> GQDEERDVGDDPFVRRAGAFLGIEAGTITIELSNLIDFYIRNGILEMENEQAVYPVNLRGVFDLNILQEMYRQYLIQSFAAKSRTEKERLFNNLAHLGNILGLTSAEVNAIHSNIGSVIYKTYASQALTNNRLEEKDIEFLRNIQNMLSMDEATCRTLLQETKEARAGFLFDKIFSRTFGMAEAVAEFRRVCRELDVDPVRDLKLTEDRRVRAFRAEIEHAIENGLITPENQSLLKESQEELGISAEKARQVLLDCIQDRCEALIVQAAASLRQRRQEGAAR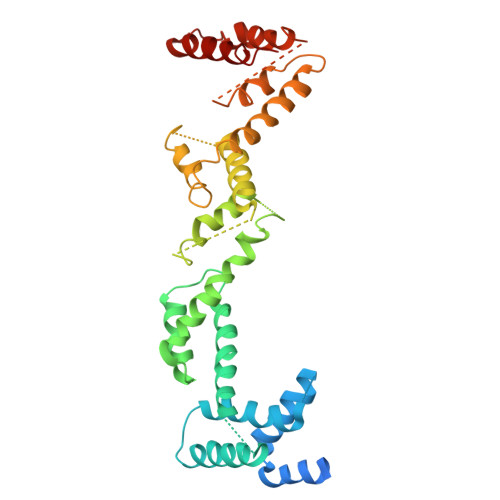DLSRALRFGKLLPFQVQTPTVTGAERQELYLVYQAYALGTARSNAENDQVKEDLALLREMLGIQAA> GNVQTTSKNDFDSRGNNGNMTFNYYANTYQNSVDFSTSS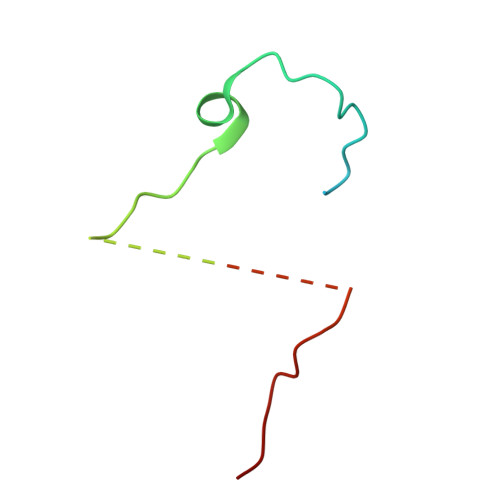SASGAGPGNSRGGLAGLLTNFSGILNPLGYLK1-methyl-5-nitro-1H-imidazole | C4 H5 N3 O2 | 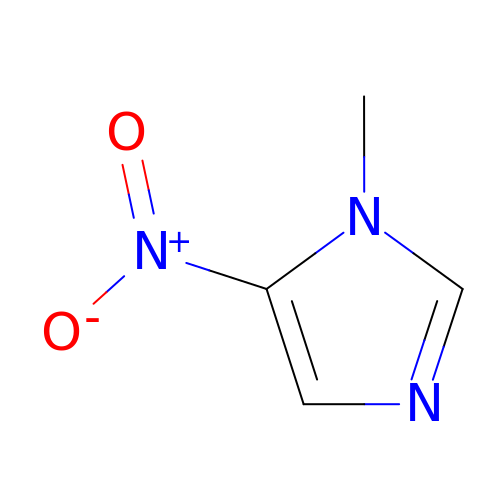JLZXSFPSJJMRIX-UHFFFAOYSA-N> MMEMITIKPGKITVQANPNMPKEVAELFRKQHYEIVGR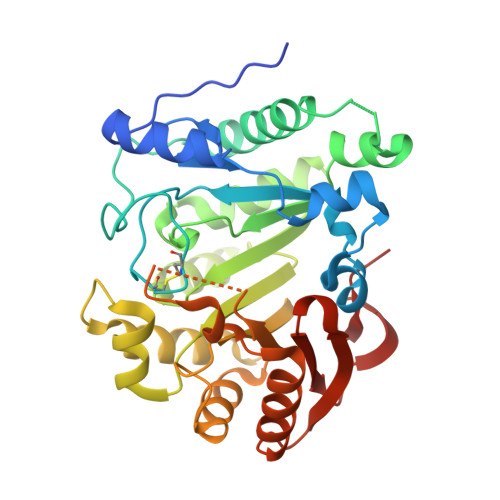HSGVKLCHWLKKSLTEGRFCYKQKFYGIHSHRCLQMTPVLAWCTHNCIFCWRPMENFLGTELPQPWDDPAFIVEESIKAQRKLLIGYKGNPKVDKKKFEEAWNPTHAAISLSGEPMLYPYMGDLVEEFHKRGFTTFIVTNGTIPERLEEMIKEDKLPTQLYVSITAPDIETYNSVNIPMIPDGWERILRFLELMRDLPTRTVVRLTLVKGENMHSPEKYAKLILKARPMFVEAKAYMFVGYSRNRLTINNMPSHQDIREFAEALVKHLPGYHIEDEYEPSRVVLIMRDDVDPQGTGVEGRFIKH> MSEIGTGFPFDPHYVEVLGERMHYVD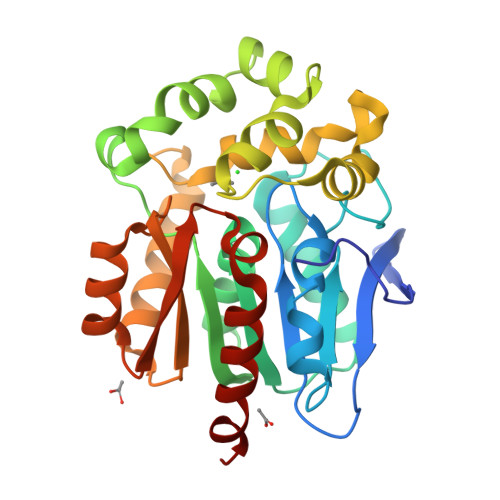VGPRDGTPVLFLHGNPTSSYLWRNIIPHVAPSHRCIAPDLIGMGKSDKPDLDYFFDDHVRYLDAFIEALGLEEVVLVIHDWGSALGFHWAKRNPERVKGIACMEFIRPIPTWDEWPEFARETFQAFRTADVGRELIIDQNAFIEGALPKCVVRPLTEVEMDHYREPFLKPVDREPLWRFPNELPIAGEPANIVALVEAYMNWLHQSPVPKLLFWGTPGVLIPPAEAARLAESLPNCKTVDIGPGLHYLQEDNPDLIGSEIARWLPALHHH> GHRP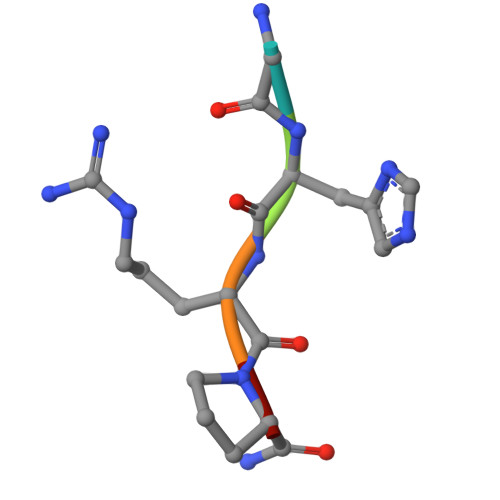X> GSMGVFTCTLADITSPVAPARLFQAFTIDNHNLMPKVVPQFVKSIDFVQGDSTAVGCVKQINFPADAPFTYVKNRVDEIDASKYYLKYTCIEGDAFPDTVEYAVYEDTFEQTETGSRCKMVAHYHLKGDSVMKEEDVAPAKEGIQKMFKAV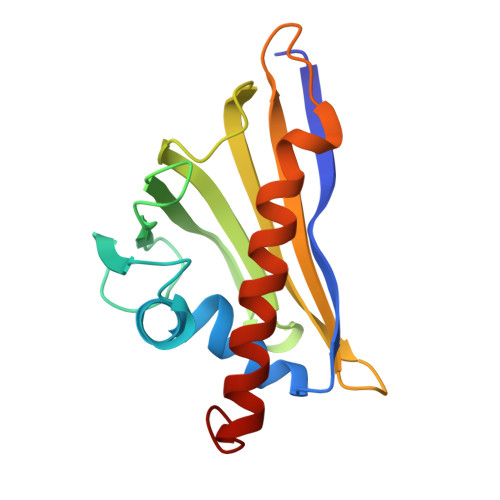EEHLIANPQLYA>[4x]GSHMTVKYTDAQIQRLREYGNGTYEQKVFEDLASRDAAFSKEMSVASTDNEKKIKGMIANPSRHGLTQLMNDIADALVAEGFIEVRTPIFISKDALARMTITEDKPLFKQVFWIDEKRALRPMLAPNLYSVMRDL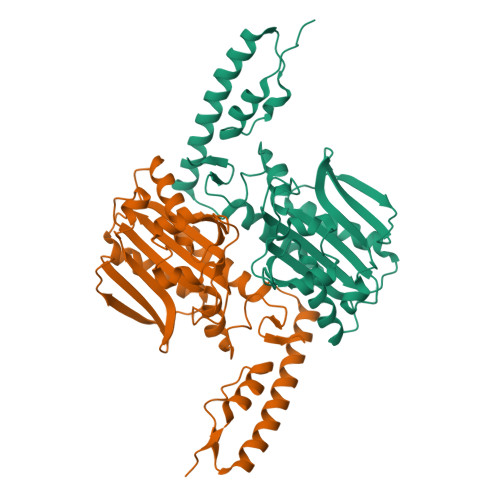RDHTDGPVKIFEMGSCFRKESHSGMHLEEFTMLNLVDMGPRGDATEVLKNYISVVMKAAGLPDYDLVQEESDVYKETIDVEINGQEVCSAAVGPHYLDAAHDVHEPWSGAGFGLERLLTIREKYSTVKKGGASISYLNGAKIN(2R)-butane-2-sulfonate | C4 H9 O3 S 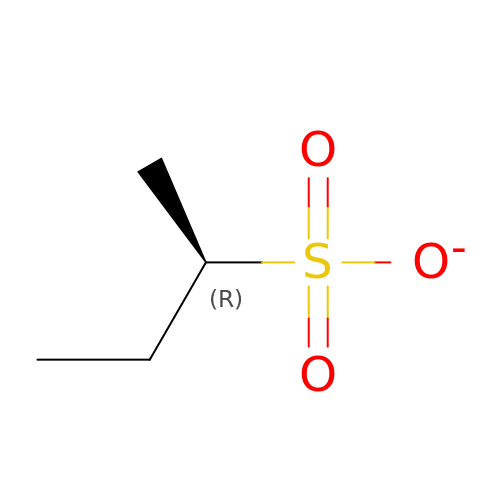| BRXCDHOLJPJLLT-SCSAIBSYSA-M>GQDMVSPPPPIADEPLTVNTGIYLIECYSLDDKAETFKVNAFLSLSWKDRRLAFDPVRSGVRVKTYEPEAIWIPEIRFVNVENARDADVVDISVSPDGTVQYLERFSARVLSPLDFRRYPFDSQTLHIYLIVRSVDTRNIVLAVDLEKVGKNDDVFLTGWDIESFTAVVKPANFALEDRLESKLDYQLRISRQYFSYIPNIILPMLFILFISWTAFWSTSYEANVTLV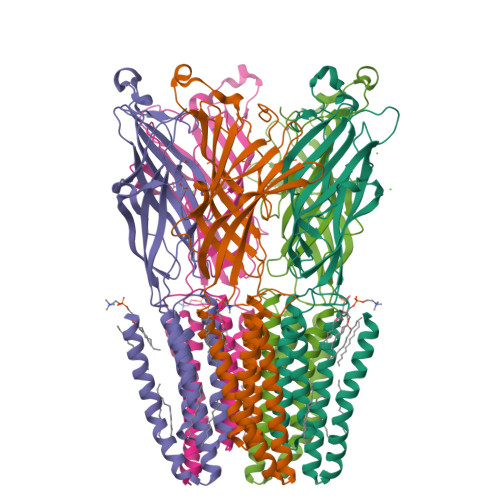VSTLIAHIAFNILVETNLPATPYMTYTGAIIFMIYLFYFVAVIEVTVQHYLKVESQPARAASITRASRIAFPVVFLLANIILAFLFFGF[5x]>[4x]GSHMASMSEVERALDVLLQEAEELCIGSSVVELDRIPTALEFCREFYSKNQPVVIRKALNWPAIGKWTPKYLIEALGDRSVDVAITPNGYAD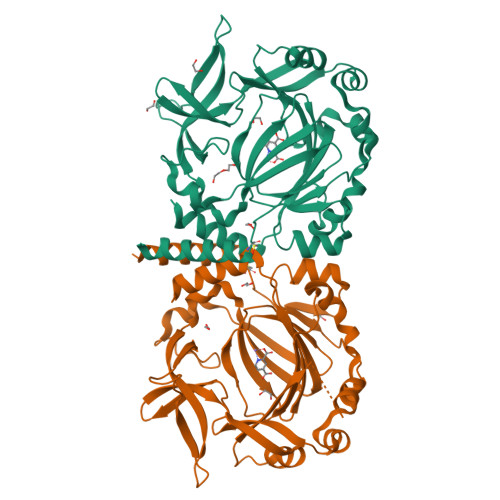GLATQNGQEYFVLPLETKMKLSEVVRRLDDPTGAVHYIQKQNSNLSVDLPELAADLRVSDLDFAQQSFNKPPDAVNFWLGDERAVTSMHKDPYENVYCVISGHKDFVLIPPHQLSCVPRGIYPTGVYKTSDSGQFYIEPLRDEEGSDQFTEWVSVDPLSPDLAKYPEYARAKPLKVRVHAGDILYLPNYWFHHVSQSHKCIAVNFWYDLDYDSRYCYYRMLEQMTSARSG> IESIIKTATDTVKSEINAELGVVPSLNAVETGATSNTEPEEAIQTRTVINQHGVSETLVENFLSRAALVS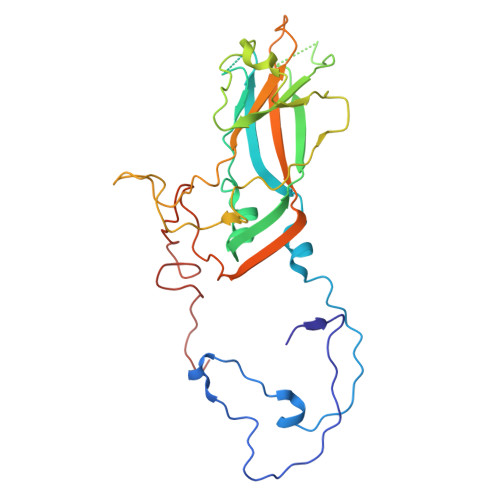KRSFEYKDHTSSAAQADKNFFKWTINTRSFVQLRRKLELFTYLRFDAEITILTTVAVNGSGNNTYVGLPDLTLQAMFVPTGALTPEKQDSFHWQSGSNASVFFKISDPPARITIPFMCINSAYSVFYDGFAGFEKNGLYGINPADTIGNLCVRIVNEHQPVGFTVTVRVYMKPKHIKAWAPRPPRTLPYMSIANANYKGKERAPNALNAIIGNRDSVKTMPHNIV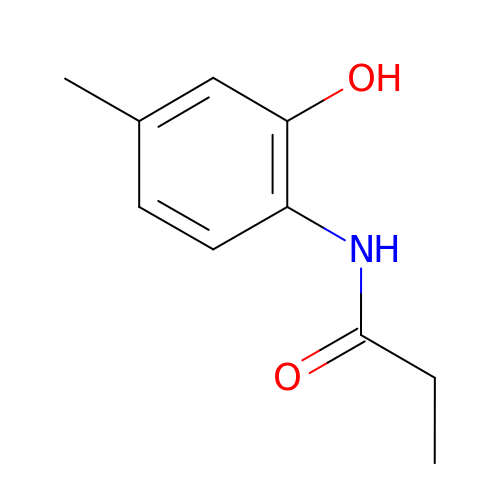~{N}-(4-methyl-2-oxidanyl-phenyl)propanamide | C10 H13 N O2 | VFXXPGGIPBIYCC-UHFFFAOYSA-N> GPGSMYSIILVALDGSQTASHALDAALELAADAHARLVPVYVVDMPVFAFDTPGYDPSILVDAFREEGRRVLDDAQARMTRRGVAGAPRLVEVEPPGEDVAERLERAAREIGASLIVMGTHGRRGVRRLMLGSVAERLLRHAR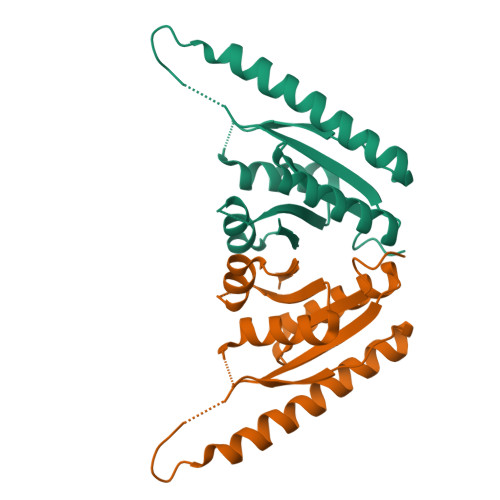CPVLMIPARGAPAADANATHPTETA>[2x]KESAAAKFERQHMDSGNSASSSSNYCNQMMCCRKMTQGKCKPVNTFVHESLADVKAVCSQKKVTCKDG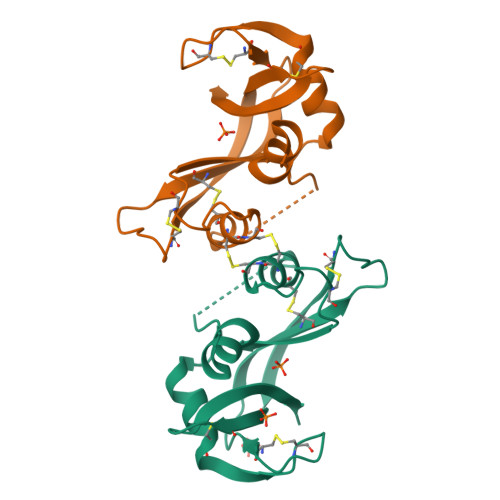QTNCYQSKSTMRITDCRETGSSKYPNCAYKTTQVEKHIIVACGGKPSVPVHFDASV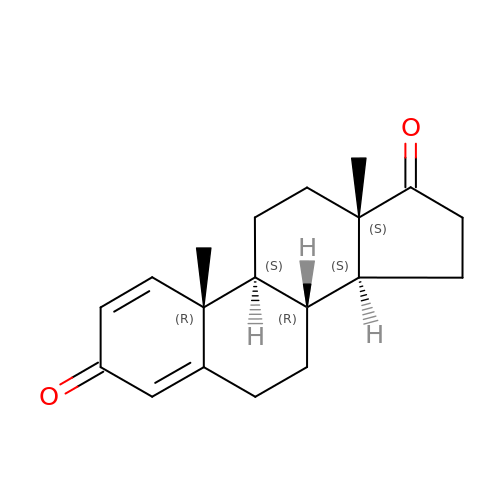ANDROSTA-1,4-DIENE-3,17-DIONE | C19 H24 O2 | LUJVUUWNAPIQQI-QAGGRKNESA-N In sequence analysis, enzyme EstDL136 was found to be a member of the HSL family. EstDL136 exhibits two different activities for the catalytic metabolism of chloramphenicol (Cm), a widely used, broad-spectrum antibiotic; it acts as both a Cm acetate esterase (CAE) and a Cm hydrolase. EstDL136 cleaves the amide linkage at C2 of Cm and thereby confers Cm resistance to bacteria heterologously expressing the EstDL136 gene. Structural analyses in this study have validated that EstDL136 contains structural features characteristic of the HSL family, with an α/β hydrolase fold and a CAP domain.

The binding of Cm to EstDL136 was achieved using the EstDL136(ΔPMP/S156A) mutant. The EstDL136(ΔPMP/S156A)‒Cm crystal also contains two monomers in the asymmetric unit. In the dimer, each monomer adopts a conformation essentially identical to that observed in EstDL136(ΔPMP), with a root-mean-square-deviation of 0.91 Å for 300 Cα atoms. Unlike other HSLs, which show ligand-induced conformational changes in the CAP region, the CAP domain of the EstDL136(ΔPMP)‒Cm complex remained identical to that of the unliganded form. Therefore, in addition to deletion of the potential hinge region in EstDL136(ΔPMP/S156A), it could be possible that extensive intersubunit interactions affect conformational mobility of the CAP region. Cm was bound to the active site of the EstDL136(ΔPMP/S156A)‒Cm complex. Specifically, the p-nitro group of Cm is located near the entrance to the active site pocket, and its C2 group points toward Ala156 located at the bottom of the pocket, a mutated residue for the catalytic residue Ser156. In particular, the CAP domain of the adjacent monomer interacts with bound Cm. Residues within 5.0 Å of the Cm-binding site include Phe34*, Ile88, His94, Asp155, Tyr205, Leu206, Phe214, and Ser286. Based on locations of those residues near the C2 group of Cm, Leu206 and Phe214 possibly facilitate a correct orientation of the C2 group toward a catalytic serine residue.

>MPLNPHVEALLQMMAQMPAPDFSVANPAEIRAVFDNLAAPPQVARVENIAISLDGRDLDARLYVPEDADERPALMVYYHGGGWVIGTLDTHDGTCRALAQKSGCAVLSIAYRLAPEYRYPAPAEDCYDALVWAKQNAATLGVDGDRLAVGGDAAGGNLAAAVAIMARDRNGPALRHQLLIYPVTDNDFTLASYAENGGGEYYLSTDGMRWFWGHYLGDTAAENAPLAAVLNVADLSGLAPATVITAEYDPLRDEGIAYAKKLDAAGVPVDAATAPGMIHGFFSMFEAVPDSWEWIERGASNLKRDLALEHHHHHHHH[2x]>[2x]MEHKRGHVLAVPYPTQGHITPFRQFCKRLHFKGLKTTLALTTFVFNSINPDLSGPISIATISDGYDHGGFETADSIDDYLKDFKTSGSKTIADIIQKHQTSDNPITCIVYDAFLPWALDVAREFGLVATPFFTQPCAVNYVYYLSYINNGSLQLPIEELPFLELQDL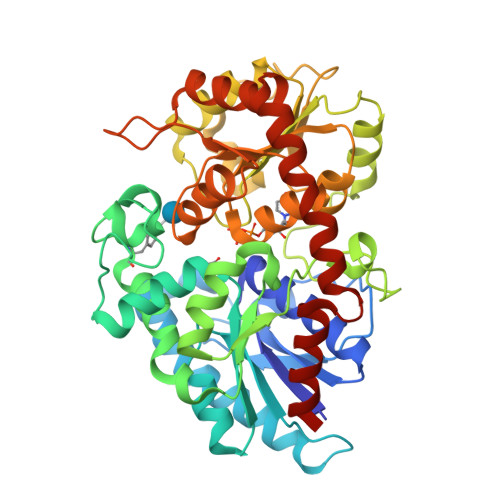PSFFSVSGSYPAYFEMVLQQFINFEKADFVLVNSFQELELHENELWSKACPVLTIGPTIPSIYLDQRIKSDTGYDLNLFESKDDSFCINWLDTRPQGSVVYVAFGSMAQLTNVQMEELASAVSNFSFLWVVRSSEEEKLPSGFLETVNKEKSLVLKWSPQLQVLSNKAIGCFLTHCGWNSTMEALTFGVPMVAMPQWTDQPMNAKYIQDVWKAGVRVKTEKESGIAKREEIEFSIKEVMEGERSKEMKKNVKKWRDLAVKSLNEGGSTDTNIDTFVSRVQSK>[4x]MSQHNEKNPHQHQSPLHDSSEAKPGMDSLAPEDGSHRPAAEPTPPGAQPTAPGSLKAPDTRNEKLNSLEDVRKGSENYALTTNQGVRIADDQNSLRAGSRGPTLLED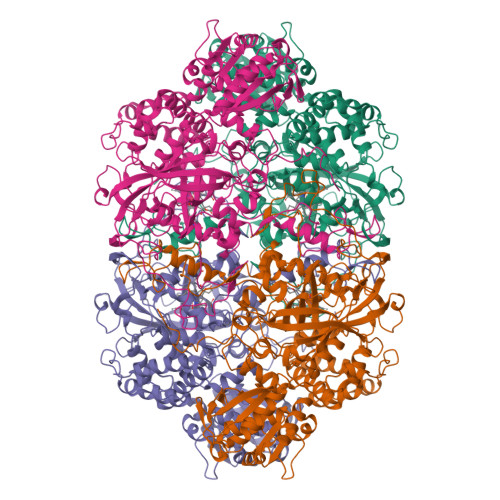FILREKITHFDHERIPERIVHARGSAAHGYFQPYKSLSDITKADFLSDPNKITPVFVRFSTVQGGAGSADTVREIRGFATKFYTEEGIFDLVGNNTPIFFIQDAHKFPDFVHAVKPEPHWAIPQGQSAHDTFWDYVSLQPETLHNVMWAMSDRGIPRSYRTMEGFGIHTFRLINAEGKATFVRFHWKPLAGKASLVWDEAQKLTGRDPDFHRRELWEAIEAGDFPEYELGFQLIPEEDEFKFDFDLLDPTKLIPEELVPVQRVGKMVLNRNPDNFFAENEQAAFHPGHIVPGLDFTNDPLLQGRLFSYTDTQISRLGGPNFHEIPINRPTCPYHNFQRDGMHRMGIDTNPANYEPNSINDNWPRETPPGPKRGGFESYQERVEGNKVRERSPSFGEYYSHPRLFWLSQTPFEQRHIVDGFSFELSKVVRPYIRERVVDQLAHIDLTLAQAVAKNLGIELTDDQLNITPPPDVNGLKKDPSLSLYAIPDGDVKGRVVAILLNDEVRSADLLAILKALKAKGVHAKLLYSRMGEVTADDGTVLPIAATFAGAPSLTVDAVIVPCGNIADIADNGDANYYLMEAYKHLKPIALAGDARKFKATIKIADQGEEGIVEADSADGSFMDELLTLMAAHRVWSRIPKIDKIPA>[2x]GALSPGGTKQKYKEVVDIEAQRRLNDLAREARIRRAQQAVLRKELIATSTNVIKSEISLRILASECHLTLNGIVEAEAQYKMGGLPKSRLPKIKHPMIVTKWVDYSNKHGFSYQLSTEDIGVLFNNGTTVLRLADAEEFWYISYDDREGWVASHYLLSEKPRELSRHLEVVDFFAKYMKANLSRVSTFGREEYHKDDVFLRRYTRYKPFVMFELSDGTFQFNFKDHHKMAISDGGKLVTYISPSHESTTYPLVEVLKYGEIPGYPESNFREKLTLIKEGLKQKSTIVTVD;>[2x]RARIERARSIEGAVQVSKGTG

Like Plks, Cdc5 contains a Ser/Thr kinase domain followed by a polo-box domain that mediates substrate recognition and sub-cellular localization. The polo-box domain is made up of two polo boxes that together define the p(S/T)-binding pocket. Cdc5 promotes the release of Cdc14 from the nucleolus and regulates the mitotic exit network (MEN)9,16–18 as well as cytokinesis. Here we demonstrate that the polo-box domain of Cdc5 uses distinct surfaces to bind phosphorylated and non-phosphorylated substrates.

Instead, it uses a unique polo-interacting motif (83RSIEGA88) to interact with the polo-box domain of Cdc527. To elucidate how Dbf4 interacts with Cdc5, we next solved the structure of the polo-box domain in the presence of a Dbf4-derived peptide (76RARIERARSIEGAVQVSKGTG96). Crystals of this complex diffracted X-rays to lower resolution (~3.5 Å), but the structure could be readily determined by molecular replacement using the polo-box domain of the Cdc5-Spc72P structure The polo-box domain was virtually identical to the other two structures (r.m.s. deviations of 0.86 and 0.66 Å with the apo- and Spc72P-bound structures, respectively). As expected, the pS/T-binding pocket was not occupied by Dbf4. After a cycle of refinement, the surface opposite to the pS/T-binding pocket showed significant peaks (>2.5σ) on the Fo-Fc electron density maps. While these additional electron densities lacked connectivity and could not account for the entire Dbf4 peptide, they could accommodate few amino acids. Intriguingly, these electron density peaks were close to the hydrophobic pocket defined by residues Leu546, Trp555, Ile557 and Ala567 from Cdc5 and coincided with the position that Phe603 occupies in the structure of the polo-box domain of Cdc5 on its own. To test whether this surface of the polo-box domain was important for the interaction with Dbf4, we introduced a A567W mutation on the polo-box domain to occlude the hydrophobic pocket. Conversely, the Dbf4 peptide failed to interact with the A567W variant of the polo-box domain, indicating that the integrity of the hydrophobic surface of the polo-box domain of Cdc5 opposite to the pS/T-binding pocket is important for Dbf4-peptide binding. Superimposition of the polo-box domain of Cdc5 onto that of zPlk1 reveals that the Dbf4-binding surface overlaps with the surface where the kinase domain binds.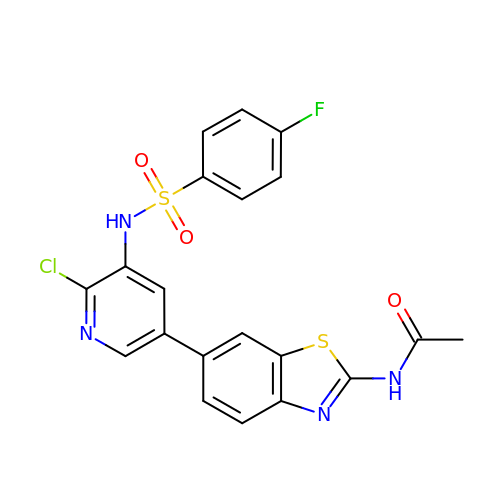N-[6-(6-chloro-5-{[(4-fluorophenyl)sulfonyl]amino}pyridin-3-yl)-1,3-benzothiazol-2-yl]acetamide | C20 H14 Cl F N4 O3 S2 | YGBMCLDVRUGXOV-UHFFFAOYSA-N> MGSSHHHHHHSQSLQEEAQGKTKKLKKVWTMLMAAKSEMADLQQEHQREIEGLLENIRQLSRELRLQMLIIDNFIPQDYQEMIENYVHWNEDIGEWQLKCVAYTGNNMRKQTPVPDKKERDPFEVDLSHVYLAYTEESLRQSLMKLERPRTSKGKARPKMGRRKRSAKPETVIDSLLQ;> MSLQQEVDIKTKKLKKLFSKLQAVKAEIHDLQEEHIKERQELEQTQNELTRELKLKHLIIENFIPLEEKNKIMNRSFFDDEEDHWKLHPITRLENQQMMKRPVSAVGYKRPLSQHARMSMMIRPEPRYRAENIMLLELDMPSRTTRDYEGPAISPKVQAALDAALQDEDEIQVDASSFESTASRKPKARPKSGRKSGSSSSSSGNPASQFYPQSRGLVPK;> MQGEDARYLKRKVKGGNIDVHPSEKALIVQYEVEATILGEMGDPMLGERKECQKIIRLKSLNANTDITSLARKVVEECKLIHPSKLSEVEQLLYYLQNRRDSLPGKEKKEKSSKPKDPPPFEGMEIDEVANINDMDEYIELLYEDIPDKVRGSALILQLARNPDNLEELLLNETALGALARVLREDWKQSVELATNIIYIFFCFSSFSHFHGLITHYKIGALCMNIIDHELKRHELWQEELSKKKKAVDEDLENQTLRKDYDKTFKKYQGLVVKQEQLLRVALYLLLNLAEDTRTELKMRNKNIVHMLVKALDRDNFELLILVVSFLKKLSIFMENKNDMVEMDIVEKLVKMIPCEHEDLLNITLRLLLNLSFDTGLRNKMVQVGLLPKLTALLGNENYKQIAMCVLYHISMDDRFKSMFAYTDCIPQLMKMLFECSDERIDLELISFCINLAANKRNVQLICEGNGLKMLMKRALKLKDPLLMKMIRNISQHDGPTKNLFIDYVGDLAAQISSDEEEEFVIECLGTLANLTIPDLDWELVLKEYKLVPFLKDKLKPGAAEDDLVLEVVIMIGTVSMDDSCAALLAKSGIIPALIELLNAQQEDDEFVCQIIYVFYQMVFHQATRDVIIKETQAPAYLIDLMHDKNNEIRKVCDNTLDIIAEYDEEWAKKIQSEKFRWHNSQWLEMVESRQLD;> MHHHHHHSQDSCISMRQSGCLPLLIQLLHGNDKDSVLLGNSRGSKEARARASAALHNIIHSQPDDKRGRREIRVLHLLEQIRAYCETCWEWQEAHEQGMDQDKNPMPAPVEHQICPAVCVLMKLSFDEEHRHAMNELGGLQAIAELLQVDCEMYGLTNDHYSVTLRRYAGMALTNLTFGDVANKATLCSMKGCMRALVAQLKSESEDLQQVIASVLRNLSWRADVNSKKTLREVGSVKALMECALEVKKESTLKSVLSALWNLSAHCTENKADICAVDGALAFLVGTLTYRSQTNTLAIIESGGGILRNVSSLIATNEDHRQILRENNCLQTLLQHLKSHSLTIVSNACGTLWNLSARNPKDQEALWDMGAVSMLKNLIHSKHKMIAMGSAAALRNLMANRPAKYKDANIMSPGSSLPSLHVRKQKALEAELDAQHLSETFDNIDNLSPKASHRSKQRHKQNLYGDYAFDANRHDDSRSDNFNTGNMTVLSPYLNTTVLPSSSSSRGSLDSSRSEKDRSLERERGIGLSAYHPTTENAGTSSKRGLQITTTAAQIA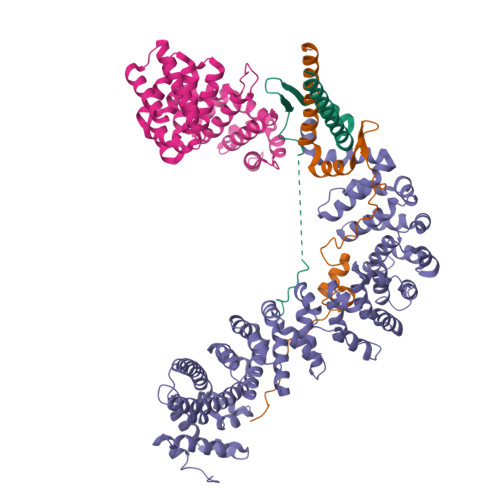KVMEEVSAIHTSQDDRSSASTTEFHCVADDRSAARRSSASHTHSNTYNFTKSENSNRTCSMPYAKVEYKRSSNDSLNSVTSSDGYGKRGQMKPSVESYSEDDESKFCSYGQYPADLAHKIHSAN> MENTENSVDSKSIKNLEPKIIHGSESMDSGISLDNSYKMDYPEMGLCIIINNKNFHKSTGMTSRSGTDVDAANLRETFRNLKYEVRNKNDLTREEIVELMRDVSKEDHSKRSSFVCVLLSHGEEGIIFGTNGPVDLKK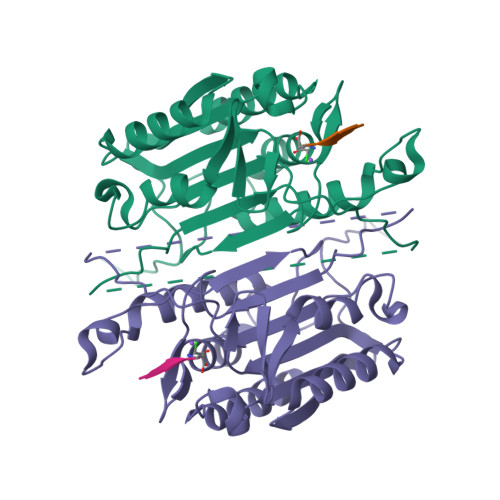ITNFFRGDRCRSLTGKPKLFIIQACRGTELDCGIETDSGVDDDMACHKIPVEADFLYAYSTAPGYYSWRNSKDGSWFIQSLCAMLKQYADKLEFMHILTRVNRKVATEFESFSFDATFHAKKQIPCIISMLTKELYFYHLH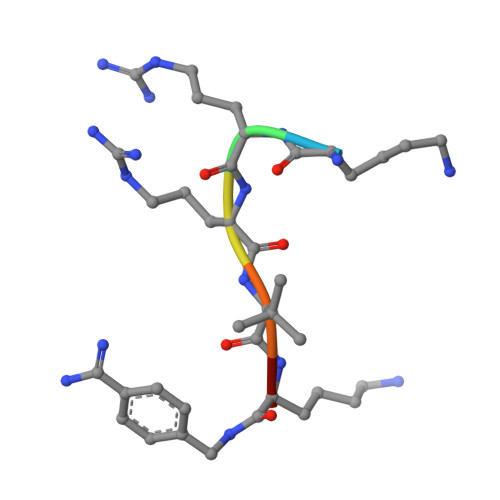> KRRVKX> MVSKRRLSKSEDKESLTEDASKTRKQPLSKKTKKSHIANEVEENDSIFVKLLKISGIILKTGESQNQLAVDQIAFQKKLFQTLRRHPSYPKIIEEFVSGLESYIEDEDSFRNCLLSCERLQDEEASMGASYSKSLIKLLLGIDILQPAIIKTLFEKLPEYFFENKNSDEINIPRLIVSQLKWLDRVVDGKDLTTKIMQLISIAPENLQHDIITSLPEILGDSQHADVGKELSDLLIENTSLTVPILDVLSSLRLDPNFLLKVRQLVMDKLSSIRLEDLPVIIKFILHSVTAMDTLEVISELREKLDLQHCVLPSRLQASQVKLKSKGRASSSGNQESSGQSCIILLFDVIKSAIRYEKTISEAWIKAIENTASVSEHKVFDLVMLFIIYSTNTQTKKYIDRVLRNKIRSGCIQEQLLQSTFSVHYLVLKDMCSSILSLAQSLLHSLDQSIISFGSLLYKYAFKFFDTYCQQEVVGALVTHICSGNEAEVDTALDVLLELVVLNPSAMMMNAVFVKGILDYLDNISPQQIRKLFYVLSTLAFSKQNEASSHIQDDMHLVIRKQLSSTVFKYKLIGIIGAVTMAGIMAADRSESPSLTQERANLSDEQCTQVTSLLQLVHSCSEQSPQASALYYDEFANLIQHEKLDPKALEWVGQTICNDFQDAFVVDSCVVPEGDFPFPVKALYGLEEYDTQNGIAINLLPLLFSQDFAKDGGPVTSQESGQKLVSPLCLAPYFRLLRLCVERQHNGNLEEIDGLLDCPIFLTDLEPGEKLESMSAKERSFMCSLIFLTLNWFREIVNAFCQETSPEMKGKVLTRLKHIVELQIILEKYLAVTPDYVPPLGNFDVETLDITPHTVTAISAKIRKKGKIERKQKTDGSKTSSSDTLSEEKNSECDPTPSHRGQLNKEFTGKEEKTSLLLHNSHAFFRELDIEVFSILHCGLVTKFILDTEMHTEATEVVQLGPPELLFLLEDLSQKLESMLTPPIARRVPFLKNKGSRNIGFSHLQQRSAQEIVHCVFQLLTPMCNHLENIHNYFQCLAAENHGVVDGPGVKVQEYHIMSSCYQRLLQIFHGLFAWSGFSQPENQNLLYSALHVLSSRLKQGEHSQPLEELLSQSVHYLQNFHQSIPSFQCALYLIRLLMVILEKSTASAQNKEKIASLARQFLCRVWPSGDKEKSNISNDQLHALLCIYLEHTESILKAIEEIAGVGVPELINSPKDASSSTFPTLTRHTFVVFFRVMMAELEKTVKKIEPGTAADSQQIHEEKLLYWNMAVR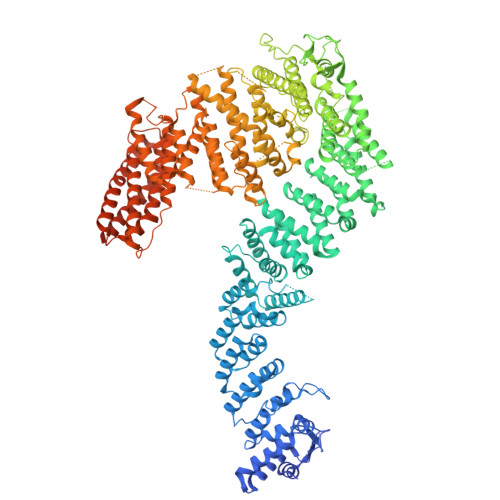DFSILINLIKVFDSHPVLHVCLKYGRLFVEAFLKQCMPLLDFSFRKHREDVLSLLETFQLDTRLLHHLCGHSKIHQDTRLTQHVPLLKKTLELLVCRVKAMLTLNNCREAFWLGNLKNRDLQGEEIKSQNSQESTADESEDDMSSQASKSKATEDGEEDEVSAGEKEQDSDESYDDSD>MRYAETGYVLEVDLTKGSIERVATDPRDTELYLGGLGTNAKILWDRVPPEVEPFSPENLLIFAAGLLCGTPATGCNRTIVSTVSPQTKLMAFSMMGGFWAPELKYAGYDKIIFRGKSPELVYLYINNDKVEIRDASHLKGKGAIETAEIIKKELNEPRAQVAAIGKAGENRVFYASIEQGRSSASRGGIGAVMGDKGLKAVVVRGTKDLCVAKPEEYIGLCNEVLDYIKHREENPIPDVMPILAGLGSPQEMKVHDEKWHTENFNWGNARTRRKDFWTDEVSHAWEKTMDKARTRLISCYNCPMKCGATISMEGLPTYMMKCFTKLTYTMAAYSDLDFGLRIAQKATEYGLDGFSAPQVMAFAFELLEKGILKDSDFPGLPEGNEERFFYLLDKIVNRDGIGDILANGTYWAAQEIGNGAEDYAHNNIKKHEQLPLKLSMLNPIYYLMYCTGEKINITQIEGQFPQAPYPKLEQREAFVEDWIQVPDEKFKKIFLEWEPRGEKSMPNFPTVDMCCDIVDWQEMMHYIDDALGQCAGLSSFPLKPPYHIHNYPKFIAAGAGIEMDTEKLKKAAKRYRTLVRAFNIRRGMRRVDEQPPANHWKNRFPELEKELLDSYYKLKGWNDDGIPTKETLDDLGLGYVGDEFIKR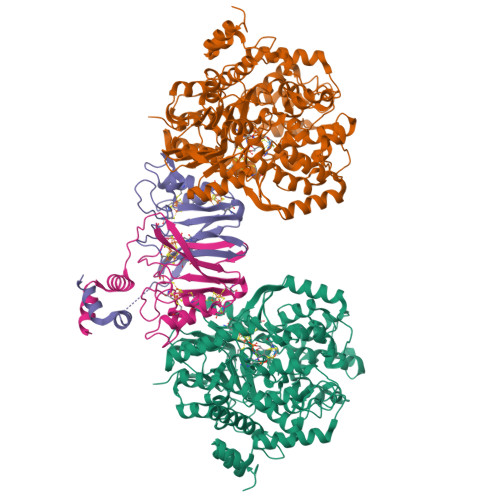GILSAG[4x];>[4x]MNSETKKRIVKTINIDADKCNGCRACEVICSAFHAMPPYSSNNPARSRVRVVRDPLRDIYVPLYAGEYTESECIGRDKFIIDGKEYDECGFCRASCPSRDLFREPDSGLPLKCDLCDGEPEPLCVKWCLVGALSVTEREVEEPDESVKRTEMEIGLESLISRFGADVVADTVEQLTKKR(2S)-4-(6-amino-9H-purin-9-yl)-2-hydroxybutanoic acid | C9 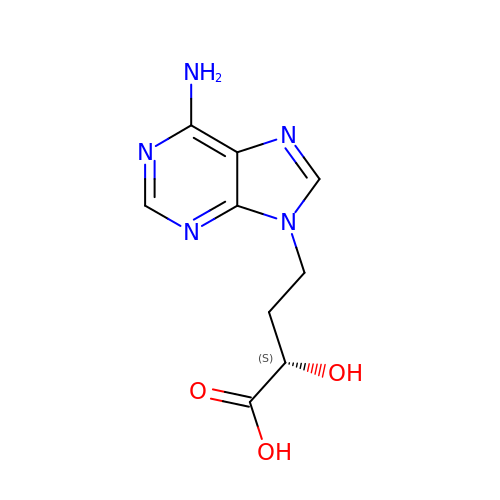H11 N5 O3 | NWPWVFAEENVVJM-YFKPBYRVSA-N>GSMPVVWPTLLDLSRDECKRILRKLELEAYAGVISALRAQGDLTKEKKDLLGELSKVLSISTERHRAEVRRAVNDERLTTIAHN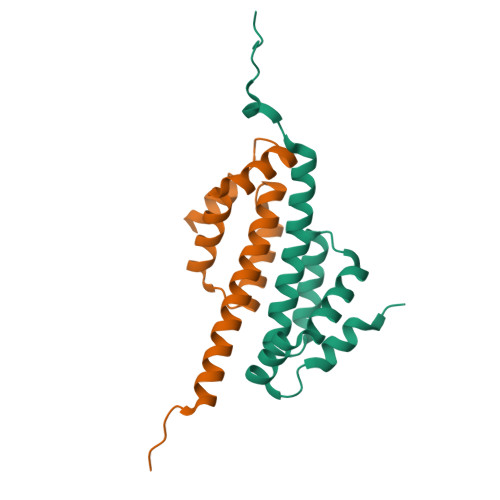MSGPNSSSEWSIEGRRLV[2x]> MATVEPETTPTPNPPTTEEEKTESNQEVANPEHYIKHPLQNRWALWFFKNDKSKTWQANLRLISKFDTVEDFWALYNHIQLSSNLMPGCDYSLFKDGIEPMWEDEKNKRGGRWLITLNKQQRRSDLDRFWLETLLCLIGESFDDYSDDVCGAVVNVRAKGDKIAIWTTECENREAVTHIGRVYKERLGLPPKIVIGYQSHADTATKSGSTTKNRFVV;> KKRYDR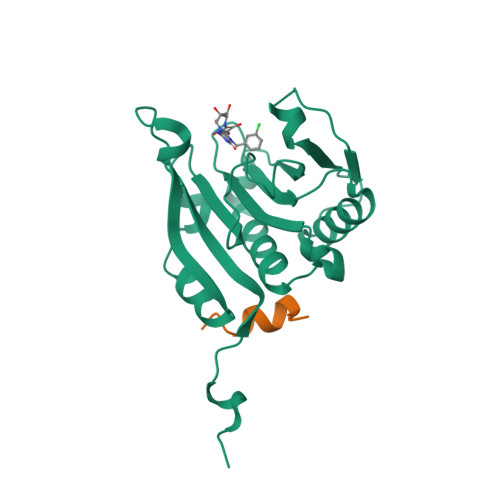EFLLGFQF> DDWRCARSMHEFSAKDIDGHMVNLDKYRGFVCIVTNVASQCGKTEVNYTQLVDLHARYAECGL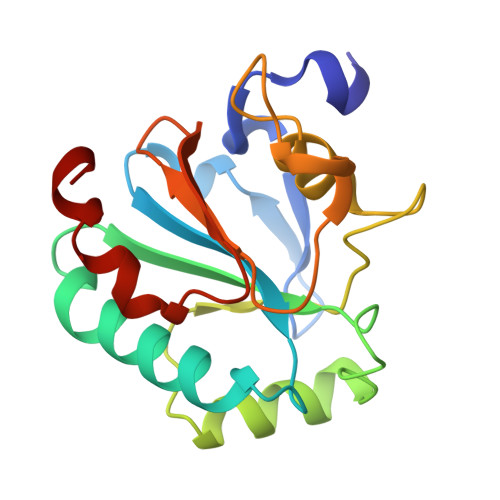RILAFPCNQFGKQEPGSNEEIKEFAAGYNVKFDMFSKICVNGDDAHPLWKWMKIQPKGKGILGNAIKWNFTKFLIDKNGCVVKHYGPMEEPLVIEKDLPHYF>[4x]GHMSTLLINQPQYAWLKELGLREENEGVYNGSWGGRGEVITTYCPANNEPIARVRQASVADYEETVKKAREAWKIWADIPAPKRGEIVRQIGDALREKIQVLGSLVSLEMGKILVEGVGEVQEYVDICDYAVGLSRMIGGPILPSERSGHALIEQWNPVGLVGIITAFNFPVAVYGWNNAIAM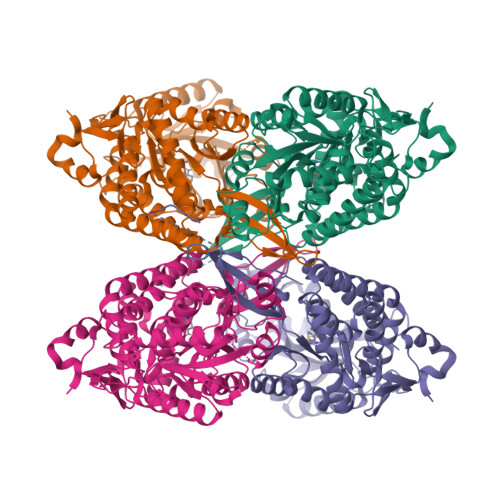ICGNVCLWKGAPTTSLISVAVTKIIAKVLEDNKLPGAICSLTCGGADIGTAMAKDERVNLLSFTGSTQVGKQVGLMVQERFGRSLLELGGNNAIIAFEDADLSLVVPSALFAAVGTAGQRCTTARRLFIHESIHDEVVNRLKKAYAQIRVGNPWDPNVLYGPLHTKQAVSMFLGAVEEAKKEGGTVVYGGKVMDRPGNYVEPTIVTGLGHDASIAHTETFAPILYVFKFKNEEEVFAWNNEVKQGLSSSIFTKDLGRIFRWLGPKGSDCGIVNVNIPTSGAEIGGAFGGEKHTGGGRESGSDAWKQYMRRSTCTINYSKDLPLAQGIKFQ> GASGDLYEVERIVDKRKNK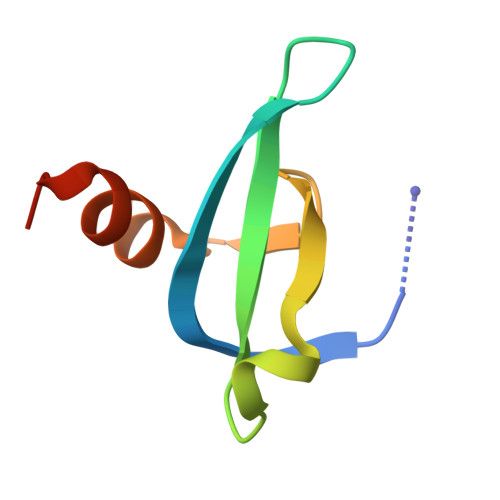KGKWEYLIRWKGYGSTEDTWEPEHHLLHCEEFIDEFNGLHMSK>[4x]MYKWSTEVGEIIIARNRDGHFYINAFVNNVKIKFMVDTGASDIALTKEDAQKLGFDLTKLKYTRTYLTANGENKAAPIT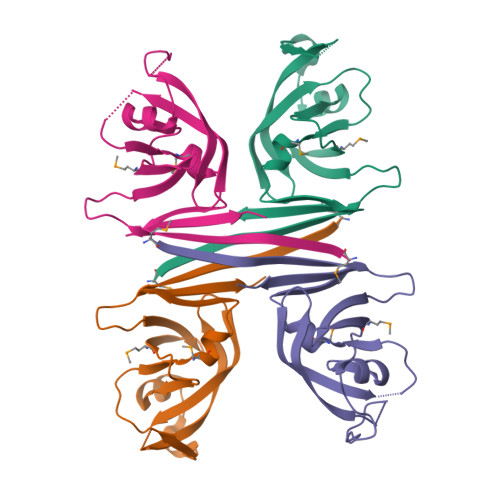LNSVVIGKEFKNIKGHVGLGDLDISLLGMSLLERFKGFRIDKDLLILNYAAALEHHHHHH>[2x]MWDERFSQSEYVYGTEPNDFLVSV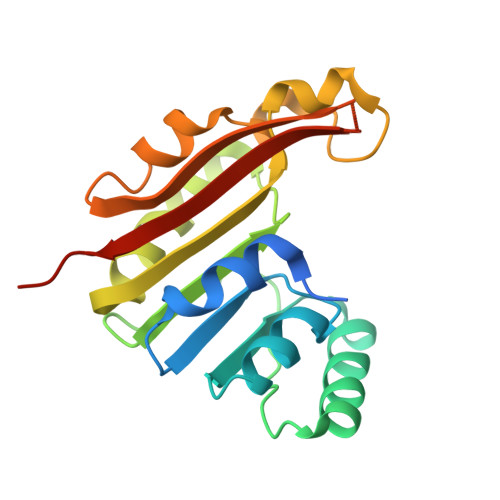ANQIPQGKILCLAEGEGRNACFLASLGYEVTAVDQSSVGLAKAKQLAQEKGVKITTVQSNLADFDIVADAWEGIVSIFCHLPSSLRQQLYPKVYQGLKPGGVFILEGFAPEQLQYNTGGPKDLDLLPKLETLQSELPSLNWLIANNLERNLDEGAYHQGKAALIQLLGQKLEHHHHHH> MAKIAQGAKYRGSIRDFPDFNPSQDAETLYNAMKGFGSDKEAIINLITSRSNKQRQEICQNYKSLYGKDLIADLKYELTGKFERLIVGLMRPPAYADAKEIKDAISGIGTDEKCLIEILASRTNEQIHQLVAAYKDAYERDLEADITGDTSGHFRKMLVVLLQGTREEDDVVSEDLVQQDVQDLYEAGELKWGTDEAQFIYILGNRSKQHLRLVFDEYLKTTGKPIEASIRGELSGDFEKLMLAVVKCIRSTAEYFAERLFKAMKGLGTRDNTLIRIMVSRSELDMLDIREIFRTKYEKSLYSMIKNDTSGEYKKTLLKLCGGDDDAAGQFFPEAAQVAYQMWELSAVARVELKGTVRPAGDFNPDADAKALRKAMKGLGTDEDTIIDIITHRSNAQRQQIRQTFKSHFGRDLMADLKSELSGDLARLILGLMMPPAHYDAKQLKKAMEGAGTDEKALIEILATRTNAEIQAINKAYKEDYHKTLEDALSSDTSGHFKRILISLATGNREEGGEDRERAREDAQVAAEILEIADTTSGDKSSLETRFMMILCTRSYPDLRRVFQEFVKMTNYDVEHTIKKEMSGDVRDVFVAIVQSVKNKPLFFADKLYKSMKG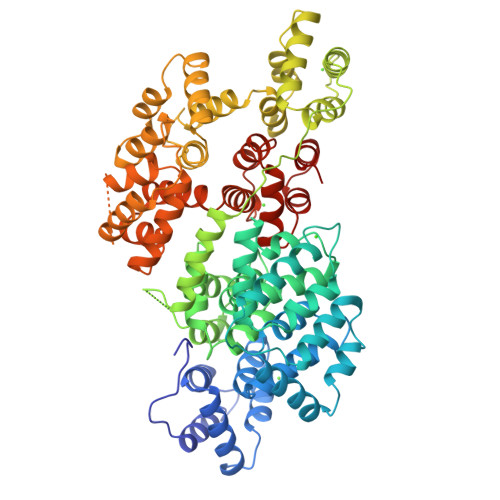AGTEEKTLTRIMVSRSEIDLLNIRREFIEKYDKSLHQAIEGDTSGHFLKALLAICGGED> MPRFAANLSMMFTEVPFIERFAAARKAGFDAVEFLFPYNYSTLQIQKQLEQNHLTLALFNTAPGDINAGEWGLSALPGREHEAHADIDLALEYALALNCEQVHVMAGVVPAGEDAERYRAVFIDN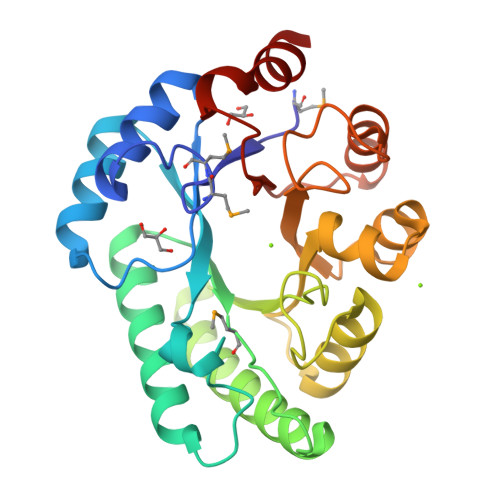IRYAADRFAPHGKRILVEALSPGVKPHYLFSSQYQALAIVEEVARDNVFIQLDTFHAQKVDGNLTHLIRDYAGKYAHVQIAGLPDRHEPDDGEINYPWLFRLFDEVGYQGWIGCEYKPRGLTEEGLGWFDAWRGS>AEPFA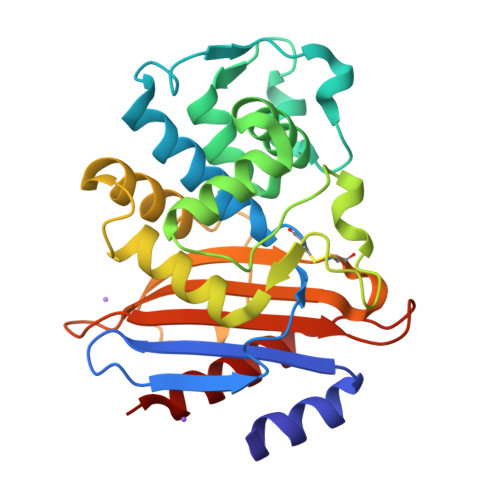KLEQDFGGSIGVYAMDTGSGATVSYRAEERFPLCSSFKGFLAAAVLARSQQQAGLLDTPIRYGKNALVPWSPISEKYLTTGMTVAELSAAAVQYSDNAAANLLLKELGGPAGLTAFMRSIGDTTFRLDRWELELNSAIPGDARDTSSPRAVTESLQKLTLGSALAAPQRQQFVDWLKGNPTGNHRIRAAVPADWAVGDKTGTCGVYGTANDYAVVWPTGRAPIVLAVYTRAPNKDDKHSEAVIAAAARLALEGLG[2x]>MIERRKIAVIGSGQIGGNIAYIVGKDNLADVV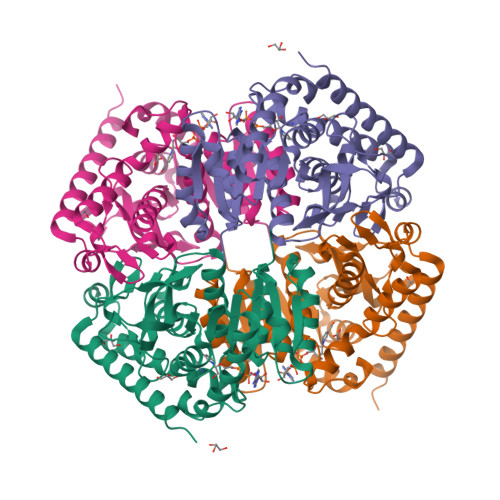LFDIAEGIPQGKALDITHSMVMFGSTSKVIGTNDYADISGSDVVIITASIPGRPKDDRSELLFGNARILDSVAEGVKKYCPNAFVICITNPLDVMVSHFQKVSGLPHNKVCGMAGVLDSSRFRTFIAQHFGVNASDVSANVIGGHGDGMVPATSSVSVGGVPLSSFIKQGLITQEQIDEIVCHTRIAWKEVADNLKTGTAYFAPAAAAVKMAEAYLKDKKAVVPCSAFCSNHYGVKGIYMGVPTIIGKNGVEDILELDLTPLEQKLLGESINEVNTISKVLDNAPAAGA[2x]> MVSVANAAQTPAAQETTKNVTIMHISTIYDKTGKATNEPALRAYDTVSVVSDPVTINNAKFYKLAGKDQYIKVGNVDGTSRTLKHNSYVYKSSGKRANKKTLKKGSSVTTYGKSFMIAGHQMYRIGKNQYVKKANFLEHHHHHH

S-layer proteins (SLPs) are self-assembling, crystalline proteins coating the cell surfaces of many prokaryotes. We determined the atomic resolution structures of all functional domains (I-III from N- to C-termini) present in the three S-layer proteins SlpA_ac, SlpX_ac, and SlpA_amy. The Lactobacillus S-layers are anchored to the cell wall through interaction with teichoic acids (TA), either lipoteichoic acid (LTA) or wall teichoic acid (WTA).

The crystal structures of the TAB domains (SlpA_ac_III, SlpA_amy_III, and SlpX_ac_III) reveal high structural similarities. The general structure of the TAB domain consists of two cell wall binding motifs (SlpA_motif) which are connected by a short linker and arranged as an internal homodimer. Mapping of the surface charges indicates a large, highly positively charged region within the interface of the two motifs that extends to the C-terminal part of the protein. SlpA_amy_III NMR chemical shift analysis of GroP trimer and GroP pentamer titrations identified two areas corresponding to phosphate-binding sites: The binding area 1 (TAB1) forms an elongated cleft in the central region of the protein, and binding area 2 (TAB2) is located in the exposed region of the C-terminal part. The main difference between the two binding regions is that both SlpA motifs contribute to the TAB1 located within the cleft of this domain. With NMR titration experiments, dissociation constants of 3.5 mM and 0.5 mM are determined for GroP trimer and GroP pentamer, respectively, indicating that longer GroP fragments increase binding strength. To obtain a molecular model of the SlpA_amy_III in complex with two GroP pentamers, we used a combination of molecular docking based on the NMR-derived chemical shift changes and classical molecular dynamics (MD) simulations. For both TAB1 and TAB2, reliable HADDOCK models were obtained and minimized in energy. Sequential analysis of TAB domains from different Lactobacillus strains (P38059, L. helveticus; A0A0PECX7L, L. gallinarum; Q09FM2 L. crispatus) reveals high conservation of residues located at the proposed TA-binding sites.> MKRPVTGKDLMIVNMGPHHPSMHGVLRLIVTLDGEDVVDCEPILGYLHRGMEKIAENRAIIQYLPYVTRWDYLATMFTEAITVNGPEQLGNIQVPKRASYIRVIMLELSRIASHLLWLGPFMADIGAQTPFFYIFREREFVYDLFEAATGMRMMHNFFRIGGIAADLPYGWIDKCLDFCDYFLTEVVEYQKLITRNPIFLERVEGVGIIGGEEAINWGLSGPMLRASGIPWDLRKIDRYESYDEFEWEIQWQKQGDSLARYLVRLSEMTESIKIIQQALEGLPGGPYENLESRGFDRKRNPEWNDFEYRFISKKPSPTFELSKQELYVRVEAPKGELGIFLIGDQSGFPWRWKIRPPGFINLQILPELVKRMKLADIMTILGSIDIIMGEVDR;> MLPMITGFMNYGQQTLRAARYIGQGFMITLSHTNRLPVTIQYPYEKLITSERFRGRIHFEFDKCIACEVCVRVCPIDLPVVDWKLETNIRKKRLLNYSIDFGICIFCGNCVEYCPTNCLSMTEEYEFSTYDRHELNYNQIALGRLPMSVIDDYTIRTIWNSPQTKNGVNPLI;> MQGTLSVWLAKRGLVHRSLGFDYQGIETLQIKPEDWHSIAVILYVYGYNYLRSQCAYDVAPGGLLASVYHLTRIEYGVNQAEEVCIKVFTHRSNPRIPSVFWVWKSTDFQERESYDMLGITYDSHPRLKRILMPESWIGWPLRKDYIAPNFYEIQDAY;> MNSIKFPILDRTTKNSVISTTLNDLSNWSRLSSLWPLLYGTSCCFIEFASLIGSRFDFDRYGLVPRSSPRQADLILTAGTVTMKMAPSLVRLYEQMPEPKYVIAMGACTITGGMFSTDSYSTVRGVDKLIPVDVYLPGCPPKPEAVIDAITKLRKKIAREIYKDRIRPQQGNRCFTTNHKFFVVRSPHIGNYDQELLYPPSSTSEISTETFFKYKSPVSSHELVN;> MSRCGSLGLYAPNALPSLSLKPRSVKSPFCITSHTKPNDTLLHNVNKMRAKACDILGAKKTILAAQLGAVLATIDHPALAITGVNNQQELSSVVLDIGIISVWYFLVMPPIIMNWLRVRWYRRKFFEMYLQFMFVFMFFPGLLLWAPFLNFRKFPRDPNMKNPWDKPTDPDSIKNVYLKYPYATPEDYDLD;> MVAAFSYTACTKLSLLHPSMVAQIRPRTTQKAFVVTNPEQDSTLEVQETETLKEEQSTEKMKKQPTPLRPVEKQLNVKSKGMGDFGGQWLSSVTRHVRIYAAYIDPETCEFDQSQMDKLTLILDPTEEFVWDDESCNKVYSYFQELVDHYEGAPLTEYTLRLIGSDVEHYIRKMLFDGEIQYNMDARVLNFSMGKPRVQFNTSNIEGGGDGQPQEDA;> MGSRAICIQRVAPPCFEASQVKKIKTVGSFLVNTR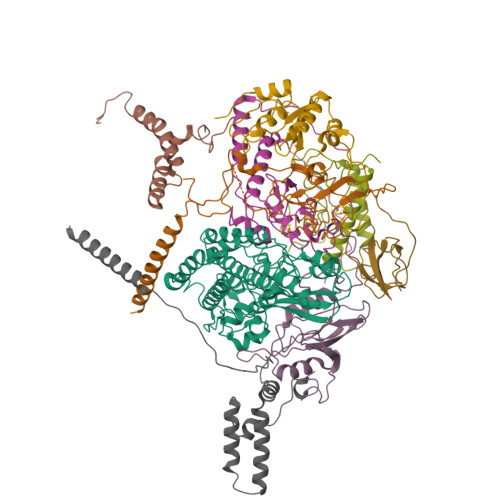SKRRRSTGVKCSSIADYIGGDLVKPDIGQWLQDVEEHKAIAIYAPHEGGYEGRYLNRLKMQGYYFLDISARGLGDPETTLLKNYPVCPAHLGKQPIARWYYPPEVDYRLAALPPSAKGLVVWVLEAKVLSKSELQFLALLPSLRPNVRVIAECGNWRKFVWKPLAEIANLAAQE;> MAFSATLSQLSSLSTISSSLPISSRRLPHRSLPQFTVKAEAEKEKQSAQAKSDGEASPAATKTPKTLPKKPVYSMKKGQIVRVEKEKYLNSINYLSVGHPPFYKGLDYIYEDRGEVLDLRVFETGEYALVGWVGIPTAPAWLPTDMLIKCEKLVYERM>GKLKVLGDVIEVGGKLKVLG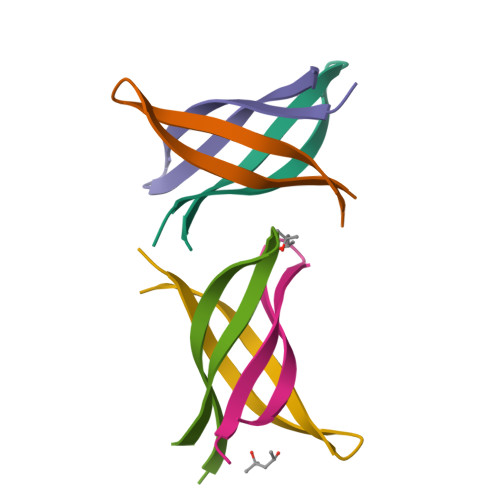DVIEV[6x]> HMQLEIQVALNFIISYLYNKLPRRRVNIFGEELERLLKKKYEGHWYPEKPYKGSGFRCIHIGEKVDPVIEQASKESGLDIDDVRGNLPQDLSVWIDPFEVSYQIGEKGPVKVLYVDDNNENGCELDKEIKNSFNPEAQVFMPISDPASSVSSSPSPPFGHSAAVSPTFMPRSTQPLTFTTATFAATKFGSTKMKNSGRSNKVARTSPINLGLNVNDLLKQKAISSSMHSLYGLGLGSQQQPQQQQQPAQPPPPPPPPQQQQQQKTSALSPNAKEFIFPNMQGQGSSTNGMFPGDSPLNLSPLQYSNAFDVFAAYGGLNEKSFVDGLNFSLNNMQYSNQQFQPVMAN

The anti-proliferative protein Tob belongs to the Tob/BTG family and plays important roles in cell proliferation, embryonic development, cellular differentiation, cancer suppression, and apoptosis. The anti-proliferative mechanism of Tob was revealed by its complex structure complex with CNOT7 (Caf1), and was further shown to be dependent on CNOT7 or CNOT8 but independent of other CCR4-NOT complex subunits. Two conserved regions of Tob, termed Box A and Box B, mediate the largely hydrophobic interaction with CNOT7 and are conserved in other family members, including BTG2. TobN138 consists of five α-helices and four β-strands that form two anti-parallel β-sheets.

To provide structural insight into fragment binding, crystals of human Tob residues 1–138 (termed TobN138 hereafter), containing Box A and B motifs, were soaked with a buffer containing several fragments. Structures of TobN138 with two inhibitors, corresponding to compounds 1 (i1) and 6 (i6), were determined to 2.3 Å resolution. The i6 complex structure revealed two inhibitor molecules from the electron density map. The first is located in the CNOT7 interface close to Box A, where i6 is coordinated by Lys63 and Asp89 and stacks loosely against His59. Superposition of Tob-i6 and Tob-CNOT7 structures shows that i6 largely overlaps with Tyr197 in CNOT7. Lys63 of Tob adopts an extended side chain conformation in the inhibitor-bound structure and would clash with Lys254 in CNOT7. Lack of sequence conservation in this site together with the low inhibition by i6 suggests it is dispensable for the CNOT7 interaction, but could be useful for design of inhibitors targeting specific Tob/BTG family members. The second inhibitor stacks against the aromatic side chain of Phe97, located on the β2-β3 loop in the Box B motif, and is further stabilized by a hydrogen bond between the O9 atom and the side chain of Glu47, in the Box A motif. Glu47 and Phe97 are strictly conserved in the Tob/BTG family, but this binding site is distant from the CNOT7 interface. The second inhibitor shows 43% inhibition and binds to a site close to Box A in the CNOT7 interface; mutation of Lys63 in this site reduces the binding affinity between Tob and CNOT7 to 47% of the wild-type.> MDEYVQELKGLIRKHIPERCEFGHQKVTFLSQVHPSPLLTEGFKLLSSLVELESCEAHACQANTDQRFVDVILSDNGILCPTLPKVIPDGFKLTGKTLILLETFVRVNPDEFEKKWKADMSKLLNLKHDLQKSGVTLVPIVDGRSNYNNRFVADWVIERIRWLLIEILKASKSMLEIDIEDQEYQRLIHSLSNVKNQSLGLENLEHLKRNSLDYDERLNESLFIGLKGDIRESTVREELIKLKLWFKDEVFSKGLGKFKLTDRRELLESLSSLGAHLDSDVSSCPFCNNKLMEIVYNVTFSCVERTDGVATVDQQFSTTHSNIEKHYLSVLSLCNKIKGLKVFNTRRNTLLFLDLIMVNLMVDISDSCQDAIESLRKSGLIVGQMVMLVNDRVLDILEAVKLIRKKIGTNPNWVKNCSKILERSHPEIWHHLSTLIKQPDFNSLISIAQHLVSDRPIMRYSVERGSDKICRHKLFQEMSSFEQMRLFKTLSSISLSLINSMKTSFSSRLLVNEREFSKYFGNVRLRECYAQRFYLAESLVGFLFYQKTGERSRCYSVYLSDNGVMSEQGSFYCDPKRFFLPVFSDEVLAGMCEEMTSWLDFDTGLMNDTGPILRLLVLAILCSPSKRNQTFLQGLRYFLMAFANQIHHIDLTSKLVVECKSSSEVVVQRLAVGLFIRLLSGESDASLFFSRRFKYLLNVSYLCHLITKETPDRLTDQIKCFEKFIEPKVKFGCAVVNPSLNGKLTVDQEDIMINGLKKFFSKSLRDTEDVQTPGVCKELLNYCVSLFNRGKLKVSGELKNNPFRPNITSTALDLSSNKSVVIPKLDELGNILSTYDKEKLVSACVSSMAERFKTKGRYNLDPDSTDYLILKNLTGLVSAGPKAKSTQEELSLMYEALTEEQVESFNEIKHDVQVALAKMADNSVNTRTKNLGRADNSVKNGNNPLDNLWSPFGVMKEIRAEVSLHEVKDFDPDVLPPEVYKELCDAVYKSSEKCNFFLEGVLDVCPLGLLLKNLTTSSYVDEEYFMCFKYLLIQGHFDQKLGSYEHKSRSRLGFTDETLRLKDEVRLSIRESNSEAIADKLDKSYFTNAALRNLCFYSEDSP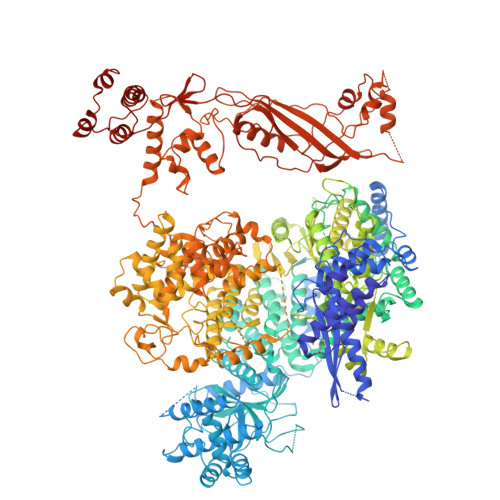TEFTSISSNSGNLKFGLSYKEQVGSNRELYVGDLNTKLMTRLVEDFSEAVGNSMKYTCLNSEKEFERAICDMKMAVNNGDLSCSYDHSKWGPTMSPALFLALLQMLELRTPVDRSKIDLDSVKSILKWHLHKVVEVPINVAEAYCIGKLKRSLGLMGCGSTSLSEEFFHQTMQLNGQIPSHIMSVLDMGQGILHNTSDLYGLITEQFLCYALDLLYDVIPVSYTSSDDQITLIKTPSLDIEGGSDAAEWLEMICFHEFLSSKLNKFVSPKSVIGTFVAEFKSRFFVMGEETPLLTKFVAAALHNVKCKTPTQLSETIDTICDQCIANGVSTKIVTRISKRVNQLIRYSGYGETPFGAIEDQDVKDWVDGSRGYRLQRKIEAIFHDDKETSFIRNCARKVFNDIKRGRIFEENLINLIGRGGDEALTGFLQYAGCSEQEVNRVLNYRWVNLSSFGDLRLVLRTKLMTSRRVLEREEVPTLIKTLQSKLSRNFTKGVKKILAESINKSAFQSSVASGFIGFCKSMGSKCVRDGKGGFLYIKEVYSGVSACTCEICALKPKIIYCNNSLNKVSQFSKPILWDYFSLVLTNACELGEWVFSTVKEPQKPLVLNNQNFFWAVKPKVVRQIEDQLGMNHVLQSIRRNYPVLFDEHLTPFMNDLQVSRTMDSGRLKFLDVCIALDMMNENLGIISHLLKTRDNSVYIVKQSDCALAHIRQSSYTDWELGLSPQQICTNFKTQLVLSSMVNPLVLSTSCLKSFFWFNEVLELEDDSQIELAELTDFALMVKNQNVSRAMFVEDIAMGYVVSNFEGVRISLSNVMVDGVQLPPQEKAPDIGELFGLKAENVIVGLVVQIDHVRMSTKFKLKRKMVYSFSLECIMDVGEIQNKEVILKVVAVDQSVSGSGGNHMLLDGVSVVASLPLFTGQASFDLAAMLIESNLAGSNDNFLMRNVTLDLGGFSPELSDKYSYRLSGPENQEDPLVLKDGAFYVGGERLSTYKVEFTGDLVVKALGALEDDESVVSMLHQLWPYLKATSQVILFQQEDFTIVHDLYKKQLTKSIESFGEWIEFTNFKVAYSKSLKELVISDTQGSFRLKGVMCRPLASTPQVEDIE> MVRYMVTSALPYANGPIHAGHLAGAYLPADIFVRYLRLKGEDVVFICGTDEHGTPISFRALKEGRSPREIVDEFHEQIKITFQRAKISFDFFGRTELPIHYKLSQEFFLKAYENGHLVKKVTKQAYCEHDKMFLPDRFVIGTCPYCGAEDQKGDQCEVCGRPLTPEILINPRCAICGRPISFRDSAHYYIKMQDFAERLKRWIEKQPWKPNVKNMVLSWIEEGLEERAITRDLNWGIPVPLDEEDMKGKVLYVWFEAPIGYISITIEHFKRIGKPNEWKKYWLNIDGQTRVIHFIGKDNIPFHAIFWPAFLMAYGKYKDEEVEAEWNLPYDIPANEYLTLEGKKFSTSRNWAIWVHEFLDVFPADYLRYYLTTIMPETRDSDFSFSDFKVRINEELVNNLGNFVHRALTFVNRYFDGVVPERGELDELDREALEEIEKAFKEVGELIMNYRFKDALKRVMSLASFGNRYFDHKQPWKTAKEDKVRTGTTVNISLQIVKALGILLEPFLPDASEKIWHLLNLDEVKRWEFRELPAGHKVRKPEILFKKVTDDQIIYFILNYMAKGNPEGARILLDKYYKREDVIRVAKEKFGDEAEVVLRRVYKDIKLKEKKEGKEMYVKFDDFAKLDL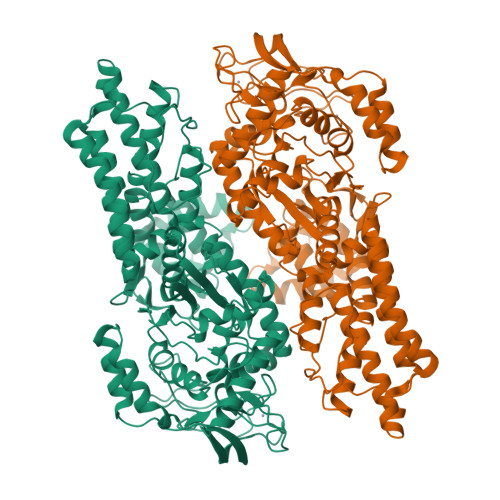RVGKIIEVKDHPNADKLYVVKVDLGDEVRTLVAGLKKYYKPEELLNRYVVVVANLEPKKLRGIGSQGMLLAADDGERVALLMPDKEVKLGAKVR alpha-D-mannopyranuronic acid 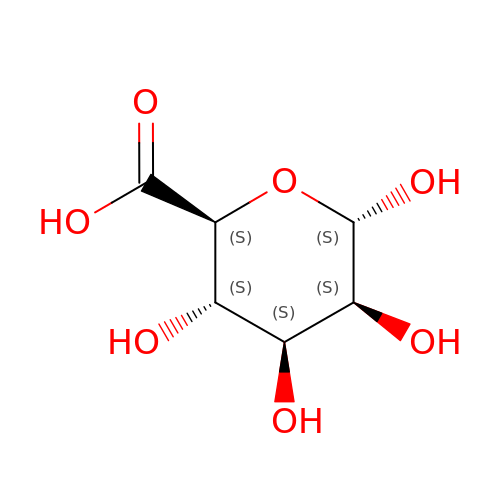| C6 H10 O7 | AEMOLEFTQBMNLQ-BYHBOUFCSA-N methyl 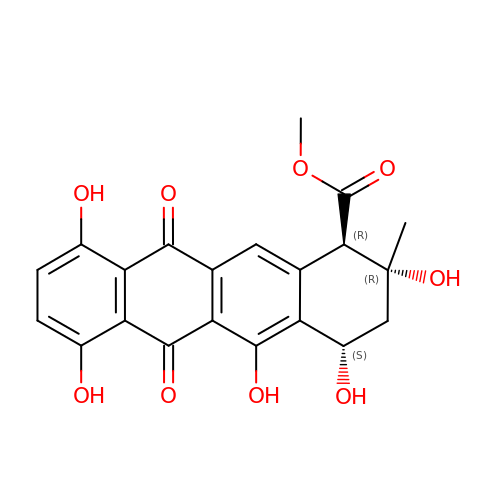(1~{R},2~{R},4~{S})-2-methyl-2,4,5,7,10-pentakis(oxidanyl)-6,11-bis(oxidanylidene)-3,4-dihydro-1~{H}-tetracene-1-carboxylate | C21 H18 O9 | ZBSRQGXAWDQXFX-SBOBAANCSA-N> ASMQKLINSVQNYAWGSKTALTELYGIANPQQQPMAELWMGAHPKSSSRITTANGETVSLRDAIEKNKTAMLGEAVANRFGELPFLFAVLCAAQPLSIQVHPNKRNSEIGFAKENAAGIPMDAAERNYKDPNHKPELVFALTPFLAMNAFREFSDIVSLLQPVAGAHSAIAHFLQVPNAERLSQLFASLLNMQGEEKSRALAVLKAALNSQQGEPWQTIRVISEYYPDDSGLFSPLLLNVVKLNPGEAMFLFAETPHAYLQGVALEVMANSDNVLRAGLTPKYIDIPELVANVKFEPKPAGELLTAPVKSGAELDFPIPVDDFAFSLHDLALQETSIGQHSAAILFCVEGEAVLRKDEQRLVLKPGESAF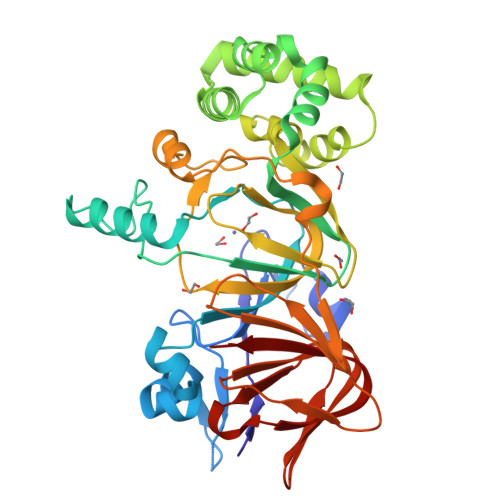IGADESPVNASGTGRLARVYNKL>[4x]MHHHHHHLPNITILATGGTIAGGGDSATKSNYTVGKVGVENLVNAVPQLKDIANVKGEQVVNIGSQDMNDNVWLTLAKKINTDCDKTDGFVITHGTTTMEETAYFLDLTVKCDKPVVMVGAMRPSTSMSADGPFNLYNAVVTAADKASANRGVLVVMNDTVLDGRDVTTTNTTDVATFKSVNYGPLGYIHNGKIDYQRTPARKHTSDTPFDVSKLNELPKVGIVYNYANASDLPAKALVDAGYDGIVSAGVGNGNLYKSVFDTLATAAKTGTAVVRSSRVPTGATTQDAEVDDAKYGFVASGTLNPQKARVLLQLALTQTKDPQQIQQIFNQY

L-asparaginases catalyze the hydrolysis of L-Asn to L-Asp. The genome of E. coli encodes three L-asparaginases, called type I, II, and isoaspartyl aminopeptidase/L-asparaginase, respectively. The active site pockets of these enzymes are shaped by two protomers, one of which forms most of the active site scaffold, including all catalytic residues; it will be referred to as a “major” protomer, with the second protomer called “minor”. Yet, as we demonstrated here based on the reinterpreted structures of EcAI and the new structures of EcAII, under some conditions a citrate ion can be accommodated into the active site cavity and even displace the canonical substrate or product.

The remaining five structures of EcAII describe its inactive variant with both Asp90 and Lys162 replaced by threonines. The remaining two structures included in this report were determined for crystals of EcAIID90T/K162T grown under the same conditions as EcAIIwt-apo7, discussed earlier. In the first case, EcAIID90T/K162T-apo7, diffraction data were collected from a crystal first transferred to the cryoprotecting solution and subsequently frozen at 100 K. For the second structure, EcAIID90T/K162T-Asn7s, a crystal was soaked for several minutes prior to freezing in the cryoprotecting solution containing 10 mM L-Asn. Both structures are isomorphous with EcAIIwt-apo7 in space group C2. The active sites are very similar for all protomers in both structures, as well as similar to protomer A in EcAIID90T/K162T-L-Asn50, described earlier. Minor differences apply to a distribution of solvent in the active site cavities and to the extent of disorder of the N-terminal hairpin. A blob of electron density was found in all active sites adjacent to the side chain of Ser58. While in the case of EcAIID90T/K162T-apo7 this density is most likely attributed to the α-carboxyl group of citrate, in the case of EcAIID90T/K162T-L-Asn50 the origin of the electron density remains uncertain.>[6x]SNAQVEFTDPEIFAEYITYPSPNGHGEVRGYLVKP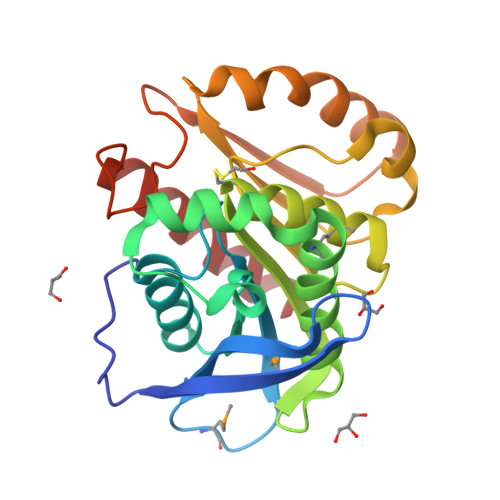AKMSGKTPAVVVVHENRGLNPYIEDVARRVAKAGYIALAPDGLNSVGGYPGNDDKGRELQQQVDPTKLMNDFFAAIEFMQRYPQATGKVGITGFCYGGGVSNAAAVAYPELACAVPFYGRQAPTADVAKIEAPLLLHFAELDTRINEGWPAYEAALKANNKVYEAYIYPGVNHGFHNDSTPRYDKSAADLAWQRTLKWFDKYL>[4x]MAAEEGAVIACHTKQEFDTHMANGKDTGKLVIIDFTASWCGPCRVIAPVFAEYAKKFP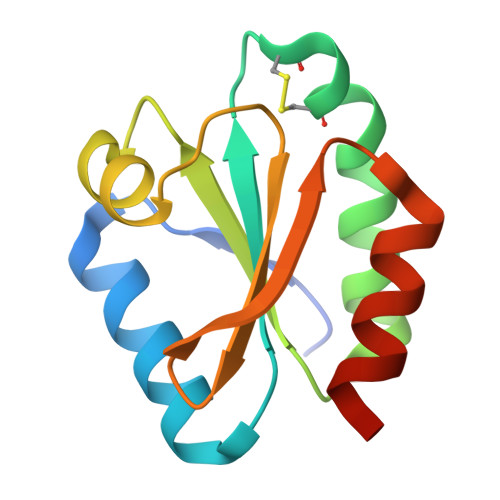GAIFLKVDVDELKDVAEAYNVEAMPTFLFIKDGEKVDSVVGGRKDDIHTKIVALMGSAST In this article, we studied five members of the PLL lectin family from P. laumondii subsp. laumondii TT01 (PLL, PLL2, PLL3, PLL4, PLL5, collectively referred to as PLLs). All studied lectins belong to the seven-bladed β-propeller structural family. Each blade makes a W-motif composed of four antiparallel beta-strands (β1-β4) connected by β-turns and loops. The saccharide binding sites are located between the adjacent blades and are uniquely organized in two separate circles around the monomer.

The newly characterized lectins PLL, PLL4, and PLL5 were produced recombinantly in Escherichia coli and were purified by affinity chromatography. The PLL chain A blade W1 interacts with chain B blade W3, whereas in the case of PLL2, PLL4 and PLL5, chain A blade W1 interacts with chain B blade W5. The PLL is a tetramer in solution (sedimentation coefficient 7.6 S); PLL4 and PLL5 form dimers in solution (sedimentation coefficients: PLL4 = 4.9 S and PLL5 = 4.7 S). PLL preferred branched fucosylated saccharides (BLeY and ALeY); PLL4 and PLL5 preferred MGMR. PLL4 also recognized linear d-fucosylated trisaccharide (d-Fucβ1-2-d-Galβ1-4-d-GlcNAcβ), α-l-fucose, and lactose. The highest affinity was seen towards methyl-α-l-fucoside (αMeFuc), ranging from 0.4 ± 0.02 mM for PLL2 to 4.9 ± 0.08 mM for PLL4. l-fucose was also significantly recognized. For PLL and PLL4, only hydrophobic site activity has been shown, as αMeFuc occupied only H sites, and structure in complex with other potential ligands is not available. However, conserved ligand binding residues in most P sites in PLL and PLL4 presume their activity.

>[2x]MQQESINTSNPDNTESYVKKDEVEIESTATGLSEIVSVANTSDGRLEVFGVGSDHAVWHNWQLTPYSNSPWSGWLSLNGNVTSKPAVYVNTDDRLEVFVRGSDNALWHNWQIAPNLGWSGWQSLGGSIASNPAVYVNTDGRLEVFVRGSDNALWHLSQTAAHSNPWSSWQSLNGNIIGNPAVHINSDGRLEVFVRGSDNALWHISQTAPDSNLWSNWESLNGSISSDPAVIGTVDGRLEVFVRGSDNALWHNWQTVPHSGPWSGWVSLNGNIISAPTVARNWDNRLEVFVCGADNALWHIWQTVSHSGPWSSWASLNGNIISAPTVAQDADGLLEVFVLGSDHALWNIRQTTSPSWSPWLSLNGSLIST> SMDRRFYG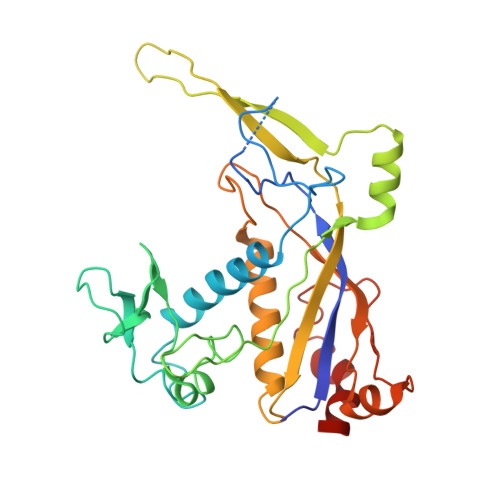KIVIKGKIKAVTGLHIGSQRDISEIGGIDNPVIKDPHTGLPYIPGSSLKGRLRSLFEILVNSRLGEWREKYPSLANYSPGSCRPDNQENCGKFFNRKINRGWIHVCPDYETALACPVCRLFGASGKESNFPSRIIVRDAFLTKEWEEKWRAGEAITEAKIEVGIDRVTSQANPRTNERVVAGAEFEFEIIYNVENTTHWRDDIKNLLTAMALLEDSYLGGSGSRGYGKVKFIFDSFEFRPLDYYRTGKDEDIVSIDAREKSVSDILSGFDSLFSEVEGKLEAG> SHMDDVYKTQPVELFYPGYLESRGYRIPALETTKKGTVLASIDVRNNGDHDAPNNNIDVGIRRKEVNGEWEEGKVILDYPGKSAAIDTSLMSATIEENGIEKERIFLIVTHFPEGYGFPNTEGGSGYKEIDGKYYFILKDAQNNEYTVREDGIVYNSEGNETDYVMKNDKTLIQNGEEVGNALLSNSPLKAVGTAHIEMIYSDDDGNTWSEPEDLNPGLKKEWMKFFGTAPGKGIQIKNGEHKGRLVFPIYYTNQNNFQSSAVIYSDDFGETWKLGESPIDTASVSSETVSSGTQLTECQVVEMPNGQLKLFMRNTGSYTR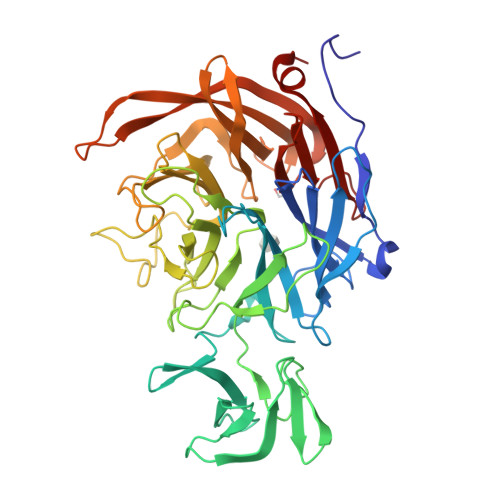IATSFDGGATWHDEVPEDTSLREPYCQLSVINYSGKINGKDAIIFSNPDASSRVNGSVKVGLINENGTYDNGEPRYEFDWIYNKTVKPGSFAYSCLTELPDGNLGLFYEGEGAGRMAYTEFDLNYLKFNA>MLRLSAPGQLDDDLCLLGDVQVPVFLLRLGEASWALVEGGISRDAELVWADLCRWVADPSQVHYWLITHKHYDHCGLLPYLCPRLPNVQVLASERTCQAWKSESAVRVVERLNRQLLRAEQRLPEACAWDALPVRAVADGEWLELGPRHRLQVIEAHGHSDDHVVFYDVRRRRLFCGDALGEFDEAEGVWRPLVFDDMEAYLESLERLQRLPTLLQLIPGHGGLLRGRLAADGAESAYTECLRLCRRLLWRQSMGESLDELSEELHRAWGGQSVDFLPGELHLGSMRRMLEILSRQALPLD[2x];>MRNDGGFLLWWDGLRSEMQPIHD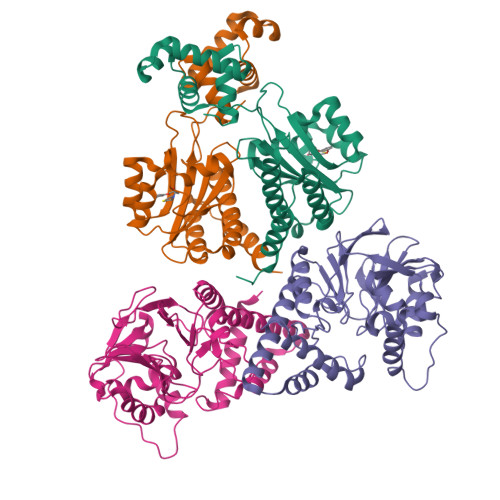SQGVFAVLEKEVRRLGFDYYAYGVRHTIPFTRPKTEVHGTYPKAWLERYQMQNYGAVDPAILNGLRSSEMVVWSDSLFDQSRMLWNEARDWGLCVGATLPIRAPNNLLSVLSVARDQQNISSFEREEIRLRLRCMIELLTQKLTDLEHPMLMSNPVCLSHREREILQWTADGKSSGEIAIILSISESTVNFHHKNIQKKFDAPNKTLAAAYAAALGLI[2x]2-chloro-1,3-benzoxazole | C7 H4 Cl N O | 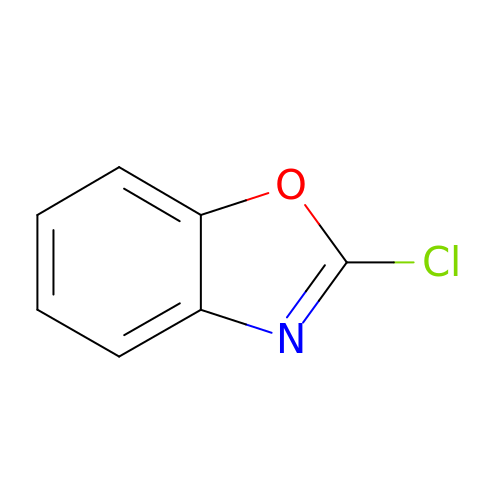BBVQDWDBTWSGHQ-UHFFFAOYSA-N>[2x]MENQEKASIAGHMFDVVVIGGGISGLSAAKLLTEYGVSVLVLEARDRVGGRTYTIRNEHVDYVDVGGAYVGPTQNRILRLSKELGIETYKVNVSERLVQYVKGKTYPFRGAFPPVWNPIAYLDYNNLWRTIDNMGKEIPTDAPWEAQHADKWDKMTMKELIDKICWTKTARRF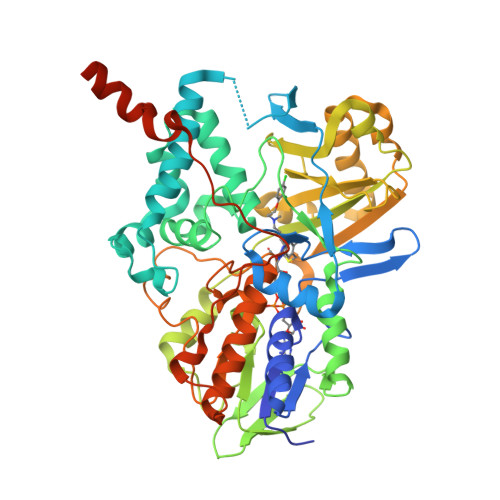AYLFVNINVTSEPHEVSALWFLWYVKQCGGTTRIFSVTNGGQERKFVGGSGQVSERIMDLLGDQVKLNHPVTHVDQSSDNIIIETLNHEHYECKYVINAIPPTLTAKIHFRPELPAERNQLIQRLPMGAVIKCMMYYKEAFWKKKDYCGCMIIEDEDAPISITLDDTKPDGSLPAIMGFILARKADRLAKLHKEIRKKKICELYAKVLGSQEALHPVHYEEKNWCEEQYSGGCYTAYFPPGIMTQYGRVIRQPVGRIFFAGTETATKWSGYMEGAVEAGERAAREVLNGLGKVTEKDIWVQEPESKDVPAVEITHTFWERNLPSVSGLLKIIGFSTSVTALGFVLYKYKLLPRS> MAETEALSKLREDFRMQNKSVFIL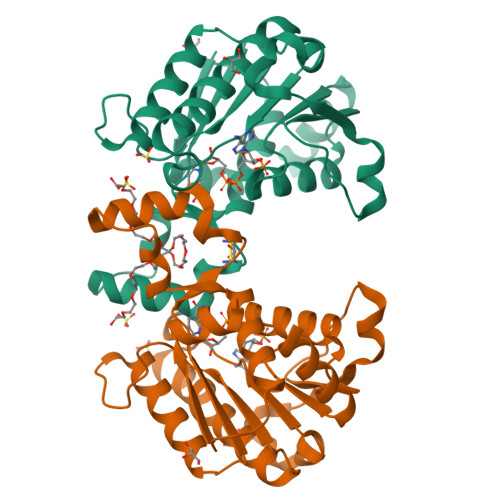GASGETGRVLLKEILEQGLFSKVTLIGRRKLTFDEEAYKNVNQEVVDFEKLDDYASAFQGHDVGFCCLGTTRGKAGAEGFVRVDRDYVLKSAELAKAGGCKHFNLLSSKGADKSSNFLYLQVKGEVEAKVEELKFDRYSVFRPGVLLCDRQESRPGEWLVRKFFGSLPDSWASGHSVPVVTVVRAMLNNVVRPRDKQMELLENKAIHDLGKAHGSLKP Acid sphingomyelinase (ASMase, ASM, SMPD1) is an enzyme found in lysosomes and in the extracellular space where it catalyses the conversion of sphingomyelin, a major component of membranes, into ceramide and phosphocholine. ASMase consists of an N-terminal saposin domain and a C-terminal catalytic domain. To gain insight into the molecular mechanism of ASMase function and the interplay between its domains, we determined crystal structures of the full-length protein from mouse that reveal a conformational flexibility of the saposin domain. In one conformation, the saposin domain adopts a globular closed form independent of the catalytic domain, while in the other conformation, it assumes an open V-shaped fold that establishes an extended interface with the catalytic domain.

We begin by describing ASMasecat, which was also crystallized in isolation. Its core, composed of two six-stranded mixed β-sheets surrounded by eight α-helices, belongs to the calcineurin-like phosphoesterase structural family (Pfam PF00149) and resembles recent structures of the ASMase-like protein, SMPDL3A. Like SMPDL3A, ASMasecat possesses an additional C-terminal subdomain (CTD) consisting of four α-helices that pack up against the core burying 1,795 Å2 of surface area, thus distinguishing it from most other phosphoesterases. In the structure of isolated ASMasecat, a phosphate ion is bound to the active site and forms several interactions with the protein and zinc ions, mimicking the scissile phosphate from sphingomyelin. As in other phosphoesterases the di-metal active site has octahedral coordination geometry from seven highly conserved protein residues, a water molecule and completed by the phosphate group. In addition, His317 and His280 are positioned near the bound phosphate as potential proton donors for the ceramide leaving group. Mutation of these histidines and assessment of enzymatic activity at acidic pH with the generic small molecule phosphodiesterase substrate bis(p-nitrophenyl) phosphate (bNPP) revealed that His280 assisted by nearby Asp249 is the likely proton donor, while His317 is probably important for substrate binding. Unexpectedly, we found that isolated ASMasecat had no activity compared with wild type, and interface mutants also diminished activity on bNPP. The structure of isolated ASMasecat is unchanged relative to the catalytic domain in the open form full-length protein, but analysis of their crystal temperature factors indicated that interface formation reduces catalytic loop dynamics.

>DRHHHHHHKLHWDIFSTWNISLPSVPKPPPKPPSPPAPGAPVSRVLFLTDLHWDHEYLEGTDPYCADPLCCRRGSGWPPNSQKGAGFWGEYSKCDLPLRTLESLLKGLGPAGPFEMVYWTGDIPAHDVWQQSRQDQLRALTTITDLVRKFLGPVPVYPAVGNHESTPVNGFPPPFIKGNQSSQWLYEAMAKAWEPWLPADALHTLRIGGFYALTPRPGLRLISLNMNFCSRENFWLLINSTDPAGQLQWLVEELQAAENRGDKVHIIGHIPPGHCLKSWSWNYYKIIARYENTLAGQFFGHTHVDEFEIFYDEETLSRPLAVAFLAPSATTFINLNPGYRVYQIDGNYPGSSHVVLDHETYILNLTQANAAGGTPSWKRLYRARETYGLPDAMPASWHNLVYRMRDDEQLFQTFWFLYHKGHPPSEPCGTPCRLATLCAQLSARADSPALCRHLMPNGSLPDANRLWSRPLLC[2x]>MADDQGCIEEQGVEDSANEDSVDAKPDRSSFVPSLFSKKKKNVTMRSIKTTRDRVPTYQYNMNFEKLGKCIIINNKNFDKVTGMGVRNGTDKDAEALFKCFRSLGFDVIVYNDCSCAKMQDLLKKASEEDHTNAACFACILLSHGEENVIYGKDGVTPIKDLTAHFRGDRCKTLLEKPKLFFIQACRGTELDDGIQADSGPINDTDANPRYKIPVEADFLFAYSTVPGYYSWRSPGRGSWFVQALCSILEEHGKDLEIMQILTRVNDRVARH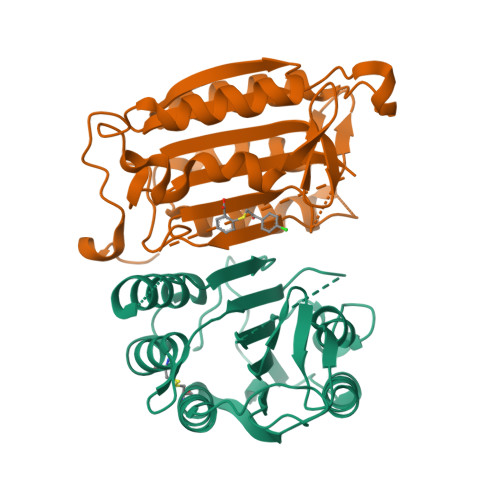FESQSDDPHFHEKKQIPCVVSMLTKELYFSQ[2x]>[4x]AVKVGINGFGRIGRNVFRAALKNPDIEVVAVNDLTDANTLAHLLKYDSVHGRLDAEVSVNGNNLVVNGKEIIVKAERDPENLAWGEIGVDIVVESTGRFTKREDAAKHLEAGAKKVIISAPAKNEDITIVMGVNQDKYDPKAHHVISNASSTTNCLAPFAKVLHEQFGIVRGMMTT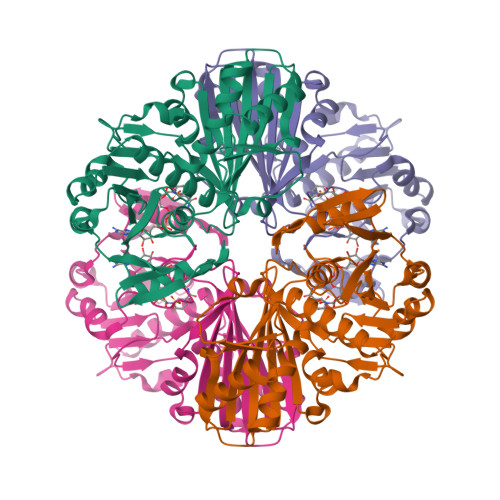VHSYTNDQRILDLPHKDLRRARAAAESIIPTTTGAAKAVALVLPELKGKLNGMAMRVPTPNVSVVDLVAELEKEVTVEEVNAALKAAAEGELKGILAYSEEPLVSRDYNGSTVSSTIDALSTMVIDGKMVKVVSWYDNETGYSHRVVDLAAYIASKGL>[2x]GPGDPHTYEDPNQAVLKFTTEIHPSCVTRQKVIGAGEFGEVYKGMLKTSSGKKEVPVAIKTLKAGYTEKQRVDFLGEAGIMGQFSHHNIIRLEGVISKYKPMMIITEYMENGALDKFLREKDGEFSVLQLVGMLRGIAAGMKYLANMNYVHRDLAARNILVNSNLVCKVSDFGLSRVLEDDPEATYTTSGGK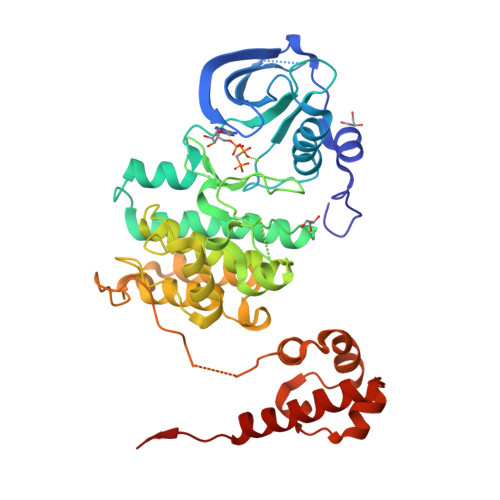IPIRWTAPEAISYRKFTSASDVWSFGIVMWEVMTYGERPYWELSNHEVMKAINDGFRLPTPMDCPSAIYQLMMQCWQQERARRPKFADIVSILDKLIRAPDSLKTLADFDPRVSIRLPSTSGEEGVPFRTVSEWLESIKMQQYTEHFMAAGYTAIEKVVQMTNDDIKRIGVRLPGHQKRIAYSLLGLKDQVNTVGIPI> MAAFVSGGCGVGGQRRAWPAKGAAVARTHACPTTMVVLPVARAGLAATAKKNQYMGTSVAPEIVLTDKGSDMSRKVKTEDKKVAADQAAAMGILANMSLYASLNPVKRMTYKAKEQAPAYVKKTGNPVEDFYPSSWRNMAPVISLSANRVAVAFEKIDAASNGVKANSNNKPFWKSGATTKNYVAPEAPAQSEPETLDDAAYQRYFPARIRNKAPAMEFRRPSFANTEDPSAYFMLQKETVPLRMALAEKLLTKLGRKGDGSEAEEEKVKPQKKAAKKDAKDDAKDDE;>[3x]MLDAFSRVVVNSDAKAAYVGGSDLQALKSFIADGNKRLDAVNSIVSNASCMVSDAVSGMICENPGLISPGGNCYTNRRMAACLRDGEIILRYVSYALLAGDASVLEDRCLNGLKETYIALGVPTNSSIRAVSIMKAQAVAFITNTATERKMSFAAGDCTSLASEVASYFDRVGAAIS

Red algae utilise a megadalton-size light harvesting antenna called the red algal phycobilisome (PBS)—comprised of rod structures formed from stacked, hexameric protein-pigment rings emanating from a protein core that is poised above an integral membrane photosystem. Published cryo-EM maps for two red algal phycobilisomes contain clusters of unmodelled density homologous to the cryptophyte-αβ protomer. We modelled these densities, identifying a new family of scaffolding proteins related to red algal phycobilisome linker proteins that possess multiple copies of a cryptophyte-α-like domain. These domains bind to, and stabilise, a conserved hydrophobic surface on phycoerythrin β, which is the same binding site for its primary partner in the red algal phycobilisome, phycoerythrin α.

We call the family of scaffolding proteins CaRSPs (CALM repeat scaffolding proteins), where each CALM domain binds a PE β, stabilising and locating it within the red algal PBS. Further inspection of the deposited maps for the P. purpureum red algal PBS revealed evidence for continuous density linking clusters of cryptophyte-like PE β subunits together; three such clusters were identified, corresponding perfectly with the three candidate CaRSP sequences that we identified from P. purpureum. The other two clusters have three and two scaffolded PE β subunits which correspond to the predicted domain architecture of the sequences that we call CaRSP1 and CaRSP2, respectively. For the unmodelled region of LR6 and most of the remaining two CaRSPs, we built de novo models including models for the metamorphic N-terminal domain of the associated PE β subunits. Analysis of each CaRSP structure confirms that they are scaffolding proteins given that two have an anchoring domain and all CaRSPs make multiple contacts with red algal PBS rods as they weave between ‘lone’ PE β subunits. Remarkably, the two CaRSP:PE β complexes in G. pacifica precisely overlay with LR6 and CaRSP1 of P. purpureum.Sestrins are a family of stress-inducible metabolic regulators that are conserved throughout the metazoan species. In addition to its antioxidant activity, Sestrins activate AMP-activated protein kinase (AMPK) and subsequently inhibit mechanistic target of rapamycin (mTOR) complex 1 (mTORC1)3. The structure of hSesn2 displays an interesting internal symmetry with two homologous subdomains (Sesn-A and Sesn-C), which have a similar structure but distinct functions. Sesn-A functions as an alkylhydroperoxide reductase, while Sesn-C performs an mTORC1-inhibiting role.

To gain insights into the biochemical and structural properties of Sestrins, we determined the crystal structure of full-length hSesn2 at 3.5-Å resolution. The electron density map of hSesn2 was calculated using the single-wavelength anomalous diffraction (SAD) method with selenomethionine (SeMet)-substituted proteins. Despite its low-resolution diffraction, we were able to obtain a high-quality electron density map by taking advantage of non-crystallographic symmetry averaging (five copies of hSesn2 per asymmetric unit (ASU)) and the high solvent content (68%). Furthermore, the helix-dominant structure and appropriately located selenium positions (total 12 sites per monomer) allowed us to precisely place the sequence in the electron density map. The crystal structure revealed that hSesn2 belongs to the family of globin-like α-helix-fold proteins, consisting of 23 helices and no β-sheets. The structure of full-length hSesn2 indicates that the protein contains three domains separated by two unstructured flexible linker regions. Although Sesn-B was originally predicted to have a coiled coil motif, it forms a helix–loop–helix structure and lies on the surface of Sesn-C. hSesn2 appears to be a monomer, both in its crystal structure as well as in its analysis using size-exclusion chromatography combined with multi-angle light scattering. Interestingly, whereas both YP_296737.1 and AhpD are characterized by a catalytic cysteine dyad (Cys86 and Cys89 in YP_296737.1), the Sesn-A domain contains only the first cysteine (Cys125 in hSesn2) with the second cysteine being substituted for a leucine (Leu128 in hSesn2). Interestingly, these two residues are located in the putative active site of Sesn-C (the helix–loop motif), indicating that Sesn-C may have acquired the mTORC1-regulating function by modifying the ancestral active site of an alkylhydroxyperoxidase during evolution.

>SNAMIVADSECRAELKDYLRFAPGGVGDSGPGEEQRESRARRGPRGPSAFIPVEEVLREGAESLEQHLGLEALMSSGRVDNLAVVMGLHPDYFTSFWRLHYLLLHTDGPLASSWRHYIAIMAAARHQCSYLVGSHMAEFLQTGGDPEWLLGLHRAPEKLRKLSEINKLLAHRPWLITKEHIQALLKTGEHTWSLAELIQALVLLTHCHSLSSFVFGCGILPEGDADGSPAPQAPTPPSEQSSPPSRDPLNNSGGFESARDVEALMERMQQLQESLLRDEGTSQEEMESRFELEKSESLLVTPSADILEPSPHPDMLCFVEDPTFGYEDFTRRGAQAPPTFRAQDYTWEDHGYSLIQRLYPEGGQLLDEKFQAAYSLTYNTIAMHSGVDTSVLRRAIWNYIHCVFGIRYDDYDYGEVNQLLERNLKVYIKTVACYPEKTTRRMYNLFWRHFRHSEKVHVNLLLLEARMQAALLYALRAITRYMT[5x]> MEALIPVINKLQDVFNTVGADIIQLPQIVVVGTQSSGKSSVLESLVGRDLLPRGTGIVTRRPLILQLVHVSQEDKRKTTGEENGVEAEEWGKFLHTKNKLYTDFDEIRQEIENETERISGNNKGVSPEPIHLKIFSPNVVNLTLVDLPGMTKVPVGDQPKDIELQIRELILRFISNPNSIILAVTAANTDMATSEALKISREVDPDGRRTLAVITKLDLMDAGTDAMDVLMGRVIPVKLGIIGVVNRSQLDINNKKSVTDSIRDEYAFLQKKYPSLANRNGTKYLARTLNRLLMHHIRDCLPELKTRINVLAAQYQSLLNSYGEPVDDKSATLLQLITKFATEYCNTIEGTAKYIETSELCGGARICYIFHETFGRTLESVDPLGGLNTIDILTAIRNATGPRPALFVPEVSFELLVKRQIKRLEEPSLRCVELVHEEMQRIIQHCSNYSTQELLRFPKLHDAIVEVVTCLLRKRLPVTNEMVHNLVAIELAYINTKHPDFADACGLMNNNIEEQRRNRLARELPSAVSRDKLIQDSRRETKNVASGGGGVGDGVQEPTTGNWRGMLKTSKAEELLAEEKSKPIPIMPASP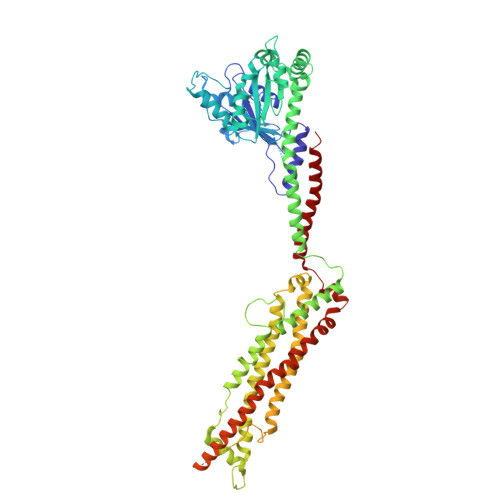QKGHAVNLLDVPVPVARKLSAREQRDCEVIERLIKSYFLIVRKNIQDSVPKAVMHFLVNHVKDTLQSELVGQLYKSSLLDDLLTESEDMAQRRKEAADMLKALQGASQIIAEIRETHLW>[4x]GPGRAPPSPDLRADEPKTPCLVGGAHAFILKISSFCGLAPLRFEPRSQEYAVTISKGKCFYSYILVTFLVICTIYGLVAEIGVGVEKSVRMSSRMSQVVSACDILVVAVTAGVGVYGAPARMRTMLSYMENIVAVDRELGRHHSAATERKLCALLLLILLSFTILLVDD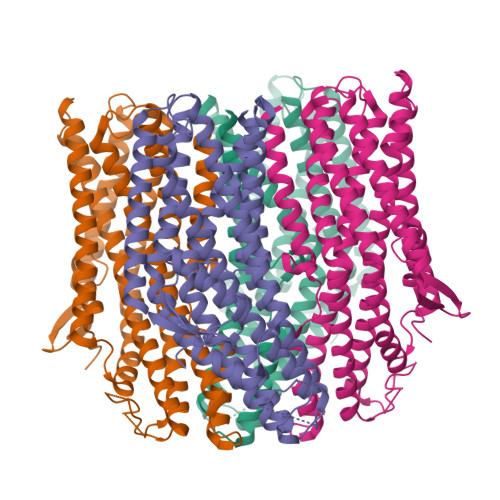FCFYAMQAGKTGRQWEIVTNYAGFYFLWYIVMVLELQFAFTALSLRARLKLFNEALNVTASQVCKPVKKPKNSQLSVYATSVRPVSCKRENVIVETIRVRDKDDAFVMMKTADGVPCLQVPPCEAVGRLSRMRCTLCEVTRHIADGYGLPLVIILMSTLLHLIVTPYFLIMEIIVSTHRLHFLVLQFLWCTTHLIRMLVVVEPCHYTIREGKRTEDILCRLMTLAPHGGVLSSRLEVLSRLLMLQNISYSPLGMCTLDRPLMVTVLGAVTTYLVILIQFQRYDS> DWVIPPISCPENEEGEFPKNLVQI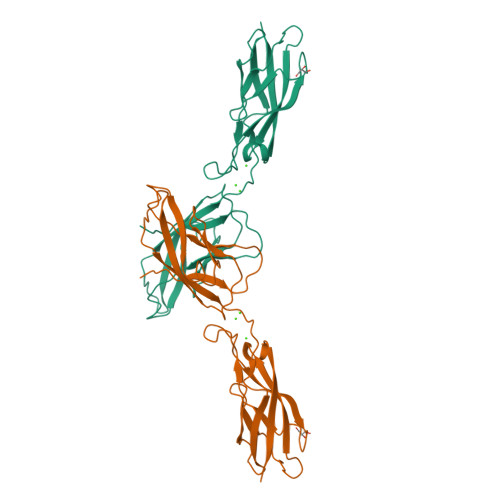KSNRDKETKVFYSITGQGADKPPVGVFIIERETGWLKVTQPLDREAIAKYILYSHAVSSNGEAVEDPMEIVITVTDQNDNRPEFTQEVFEGSVAEGAVPGTSVMKVSATDADDDVNTYNAAIAYTIVSQDPELPHKNMFTVNRDTGVISVLTSGLDRESYPTYTLVVQAADLQGEGLSTTAKAVITVKD> MGSSHHHHHHSQDPAGGNWTVFDEVLDSNVIKQLTLTGCGAACGEMLLRD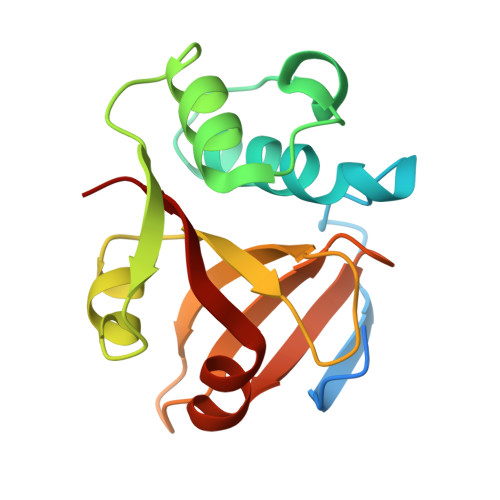RYIFVTQNVIGTELTSMTSLANKLNKFDVGWEGNAVSESSLYALSNTGSWGAMMWDSGSKVGHWVLVKGVDDAGNVIIYDPYQGSRYLMTEQEFKEVWNGHSVYKP>GSHMNGKLKWKFETGGS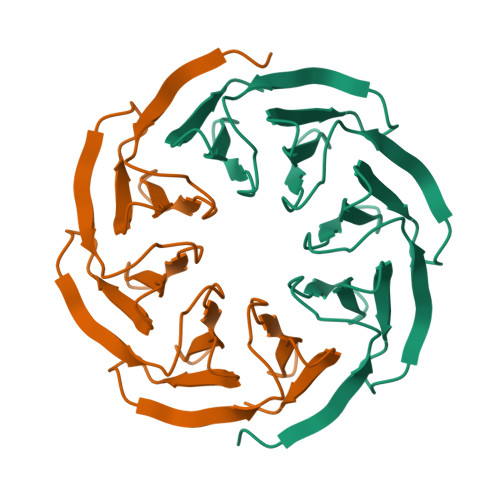VHSSPAIGQDGTIYVGSNDHYLYAINPNGKLKWKFETGGSVHSSPAIGQDGTIYVGSNDHYLYAINPNGKLKWKFETGGSVHSSPAIGQDGTIYVGSNDHYLYAINPNGKLKWKFETGGSVHSSPAIGQDGTIYVGSNDHYLYAINPG[4x]(2R,4S)-N-butyl-4-[(2S,5S,7R)-2,7-dimethyl-3,15-dioxo-1,4-diazacyclopentadecan-5-yl]-4-hydroxy-2-methylbutanamide 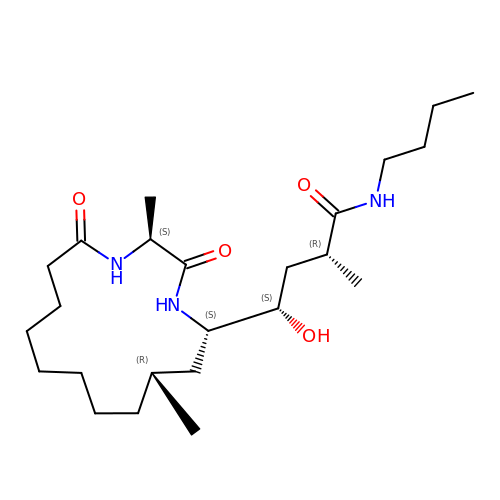| C24 H45 N3 O4 | ZUIGWVKXPZANDI-MJCUULBUSA-N> MFPEVVELNVGGQVYFTRHSTLISIPHSLLWKMFSPKRDTANDLAKDSKGRFFIDRDGFLFRYILDYLRDRQVVLP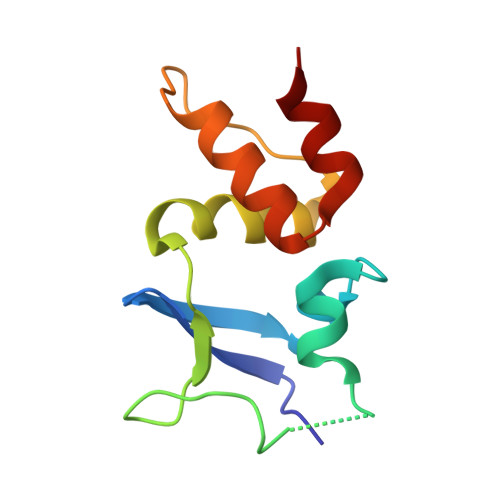DHFPEKGRLKREAEYFQLPDLVKLLTP(1R,4S,5R)-3-(BENZO[b]THIOPHEN-5-YL)METHOXY-2-(BENZO[b]THIOPHEN-5-YL)METHYL-1,4,5-TRIHYDROXYCYCLOHEX-2-ENE-1-CARBOXYLATE | C25 H22 O6 S2 | 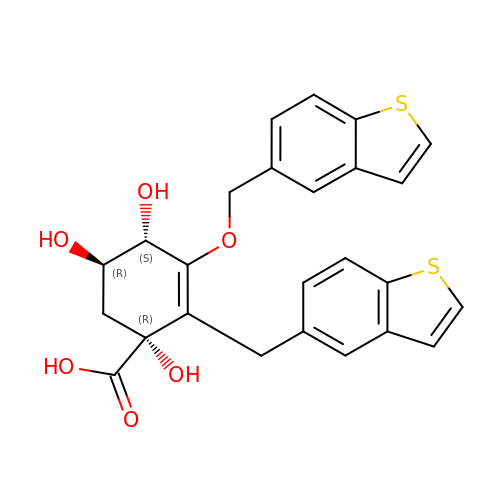MGSLLSIRNDMRFT-RZTXVSJASA-N>[4x]MSQSSRLSALPIFQASLSASQSPRYIFSSQNGTRIVFIQDNIIRWYNVLTDSLYHSLNFSRHLVLDDTFHVISSTSGDLLCLFNDNEIFVMEVPWGYSNVEDVSIQDAFQIFHYSIDEEEVGPKSSIKKVLFHPKSYRDSCIVVLKEDDTITMFDILNSQEKPIVLNKPNNSFGLDARVNDITDLEFSKDGLTLYCLNTTEGGDIFAFYPFLPSVLLLNEKDLNLILNKSLVMYESLDSTTDVIVKRNVIKQLQFVSKLHENWNSRFGKVDIQKEYRLAKVQGPFTINPFPGELYDYTATNIATILIDNGQNEIVCVSFDDGSLILLF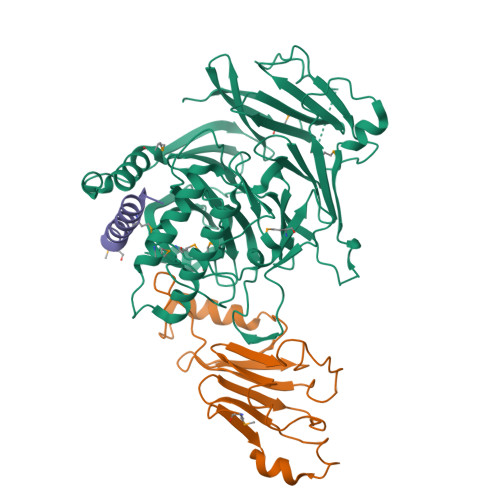KDLEMSMSWDVDNYVYNNSLVLIERVKLQREIKSLITLPEQLGKLYVISDNIIQQVNFMSWASTLSKSINESDLNPLAGLKFESKLEDIATIERIPNLAYINWNDQSNLALMSNKTLTFQNISS;>MNENYYISPSLDTLSSYSLLQLRKVPHLVVGHKSYGKIEFLEPVDLAGIPLTSLGGVIITFEPKTCIIYANLPNRPKRGEGINVRARITCFNCYPVDKSTRKPIKDPNHQLVKRHIERLKKNPNSKFESYDADSGTYVFIVNHAAEQT[4x];>SSITKDMKGFKVVEVGLAMNTKKQIGDFFKNLNMAK[4x]>[2x]MGHHHHHHGSPEDLSLEEREELLDIRRRKKELIDDIERLKYEIAEVMTEIDNLTSVEESKYTQRNAQIAMGRKKFNMDPKKGIQFLIENDLLQSSPEDVAQFLYKGEGLNKTVIGDYLGERDDFNIKVLQAFVELHEFADL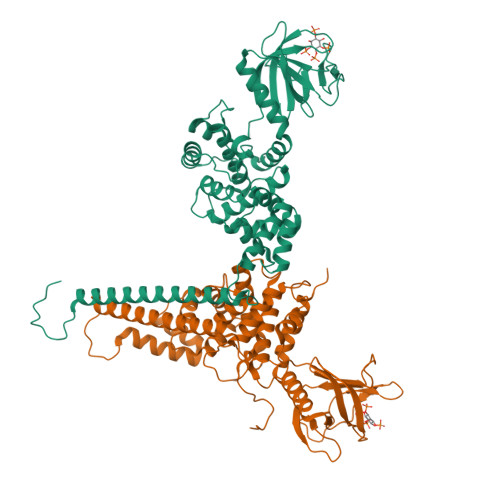NLVQALRQFLWSFRLPGEAQKIDRMMEAFASRYCLCNPGVFQSTDTCYVLSFAIIMLNTSLHNHNVRDKPTAERFITMNRGINEGGDLPEELLRNLYESIKNEPFKIPEDDGNDLTYTFFNPDREGWLLKLGGRVKTWKRRWFILTDNCLYYFEYTTDKEPRGIIPLENLSIREVEDPRKPNCFELYNPSHKGQVIKACKTEADGRVVEGNHVVYRISAPSPEEKEEWMKSIKASISRDPFYDMLATRKRRIANKK7-[2-[2-(3-fluorophenyl)ethylamino]ethyl]quinolin-2-amine | 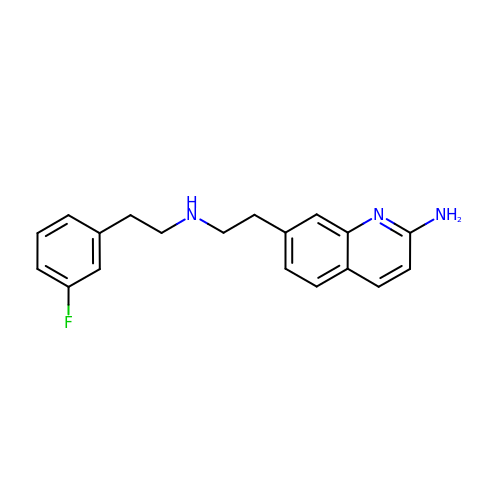C19 H20 F N3 | UAVGQDSBRIPETE-UHFFFAOYSA-N> GAGCA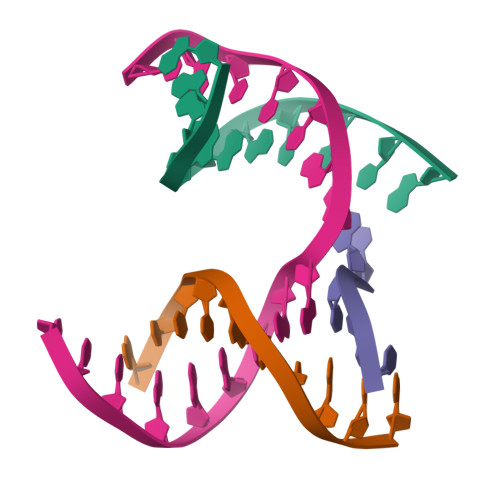GACTTG;> ACACCACTCA;> CATGT;> TCTGAGTGAGGTCTGC>MISDAMRLIQVALQRYILEFEPELGLSQVVIIENIAMAEELGGQNNQINGHVVMSLVNLQEETTLKNSPHYRLDNGRTIYQNPPVNLNLFILFSALHNQYETSLRLLSRVVEFFQWQKELSFTTTPGIGGISRDLRILPDLYSLTFEQLNHLWGALGGKQVPFVLYRARILSLEAPKRQAEGSTITEIYINE[6x];>MKILYKKILNLELWHDFYLGQPNTPGSLPNNYDISRTLALVPTQECLRVLANLRWVFRPQLYGASLFANVNAAPSGQFPTIFPIDRVYRLTFWLVVSDRYFANFTNLSLINSRNQIYYFSNLSGNEGHALFLTQPLSAYTTNNEYQLGQLVTHADKTLESL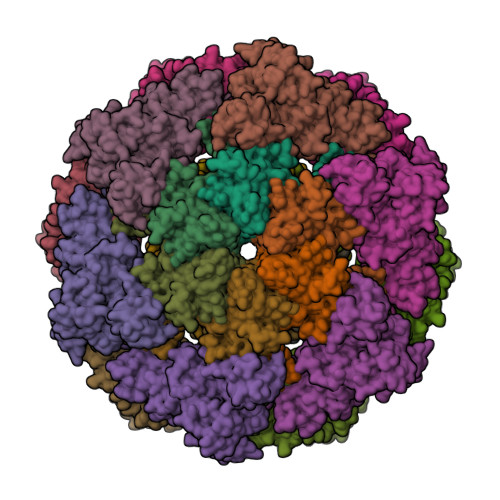TYQGNATNIPNPSDWDSLPASQYVSELDHLPRQGTYRTQVITNANPDNTYNFTLVNTNEQESWAIDVIVPDTHKSGEPFSTSLNFVGQTPGHYRLLENDTQVAEFVLVDNSLPEAFALVEVILNPELVPSAFSLLQASAGQTFIQPKTYVIRFKNRATRWRYRYEQPHGCSAANLPSYFNLIDTHTYATARPIGLRQRPDSLLNDCQDRPLPAPSITLIQPETDGSQRIARIFSDIYL[6x];>MPSTYKTPGVYIEEISKFPPSIAQVETAIPAFIGYTQIAKVGVENFHTDADNLILRPVRITSLLEYEQFFGKAINETTIQVVIQDTTDSRGNLTERKASARITSPSPHNLYYSMQAYFANGGGPCYIVSVGPMSNTGTIQLEALQNGLAEVAKEDEVTLLVFPESQSLSDENYAALMSAALEQCANLQDRFTVMDLKLPATRPIPANAIVGASNAFRDLSLPQDNLKYGACYAPDIETIFNYFYQEDAVTIFRSVNGGAEEQDTLTMAGYNPANGGDGIQYALIESAIDQLPLILPPSPLVVGQYARTDNTRGVWKAPANVALSSVIKPVLKITNEQQNNLNVHPTGKSINAIRAFTGKGTLIWGARTLAGNDNEWRYVSVRRFFNMAEESIKKGSEPFVFEPNDANTWTKVKAMIENFLTLQWRAGALAGAKPEQAFYVKIGLNETMTALDILEGRMIVEIGMAVVRPAEFIILKFSHKMQES[6x];>MAEYPLPKFHFQVDWGGSRLGFTEVSGLDVETEVIEYREGNLPQYHKLKMPGMQKFSNITMKRGTFQGDNDFYKWWNTVALNTIERRDLTISLLNEKHEPVVVWKVNRAWPTKVQSTDLKGDGNEVAIESIEVAHEGLTIQNG[12x]> MLAKRIIACLDVKDGRVVKGSNFENLRDSGDPVELGKFYSEIGIDELVFLDITASVEKRKTMLELVEKVAEQIDIPFTVGGGIHDFETASELILRGADKVSINTAAVENPSLITQIAQT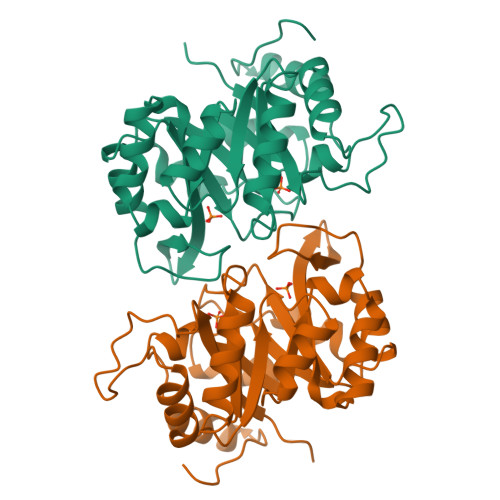FGSQAVVVAIDAKRVDGEFMVFTYSGKKNTGILLRDWVVEVEKRGAGEILLTSIDRDGTKSGYDTEMIRFVRPLTTLPIIASGGAGKMEHFLEAFLAGADAALAASVFHFREIDVRELKEYLKKHGVNVRLEGL>RGSHMMFVHIADNHLGYRQYNLDDREKDIYDSFKLCIKKILEIKPDVVLHSGDLFNDLRPPVKALRIAMQAFKKLHENNIKVYIVAGNHEMPRRLGEESPLALLKDYVKILDGKDVINVNGEEIFICGTYYHKKSKREEMLDKLKNFESEAKNYKKKILMLHQGINPYIPLDYELEHFDLPKFSYYALGHIHKRILERFNDGILAYSGSTEIIYRNEYEDYKKEGKGFYLVDFSGNDLDISDIEKIDIECREFVEVNIKDKKSFN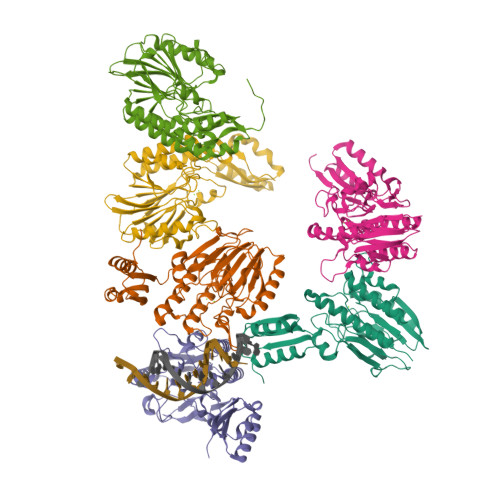EAVNKIERCKNKPVVFGKIKREFKPWFDTLKDKILINKAIIVDDEFIDMPDNVDIESLNIKELLVDYANRQG[6x]>[4x]SGSMTSSNRITSPAMTASKTAAVAKPTRAGRKAPAVETAPEASELKMGELSELLGYALKRAQLRVFEDFLHCVAPVQLTPAQFSVLLLLDANPGRN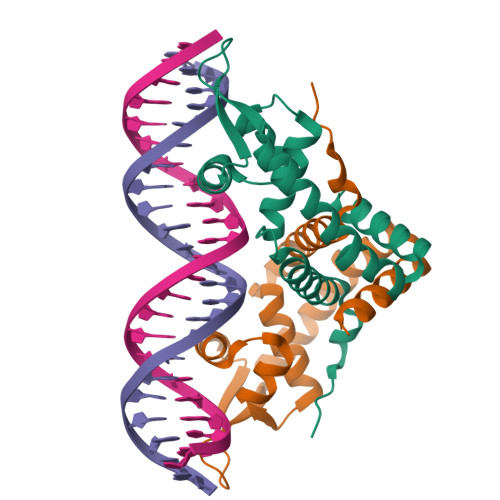QTEIATTLGILRPNFVAMLDALEGRGLCVRTRSPSDRRSHILMLTDKGRATLARAKKLVATRHEDRLTELLGRDNRDALLSMLATIAREF1-[4-(trifluoromethyloxy)phenyl]thiourea 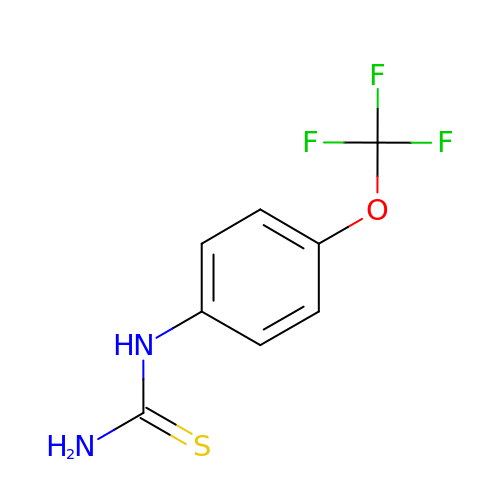| C8 H7 F3 N2 O S | UCOXNOVULREFCO-UHFFFAOYSA-N> PFEW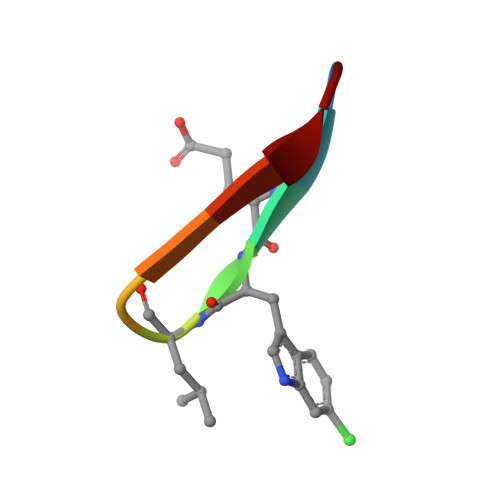LDWEFP>HMIEPVLENVQPNSAASKAGLQAGDRIVKVDGQPLTQWVTFVMLVRDNPGKSLALEIERQGSPLSLTLIP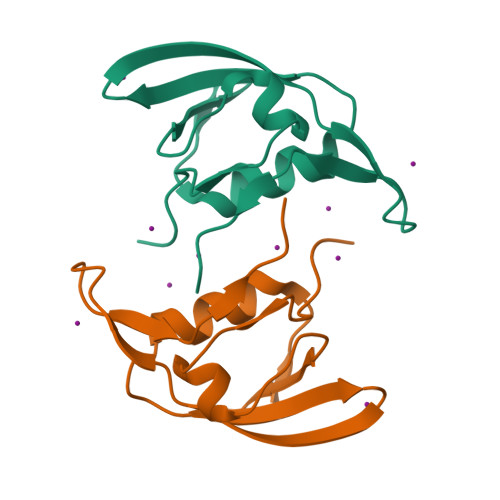ESKPGNGKAIGFVGIEPKVI[2x]>GSHMRVQVSGLSDETTWHTLKDHLRQAGEVTFCKVFSGGRAVVEFVTPED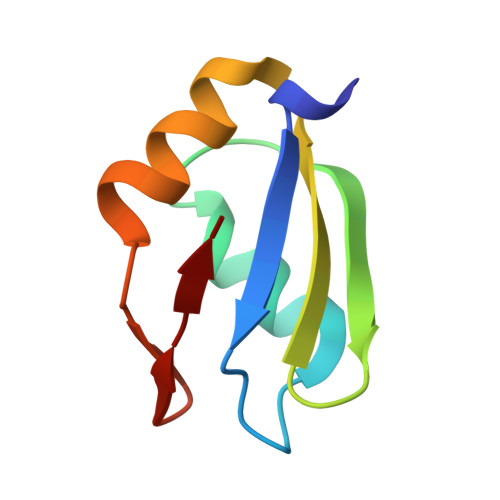AARAITELQASELEGATLFLR[4x]>MALKMLTRLQVLTLALFSKGFLLSLGDHNFLRREIKIEGDLVLGGLFPINEKGTGTEECGRINEDRGIQR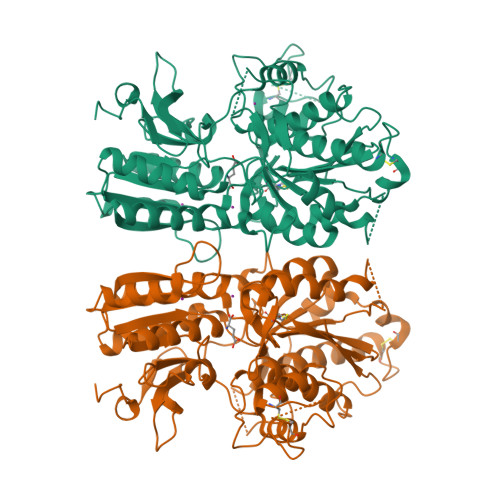LEAMLFAIDEINKDDYLLPGVKLGVHILDTCSRDTYALEQSLEFVRASLTKVDEAEYMCPDGSYAIQENIPLLIAGVIGGSYSSVSIQVANLLRLFQIPQISYASTSAKLSDKSRYDYFARTVPPDFYQAKAMAEILRFFNWTYVSTVASEGDYGETGIEAFEQEARLRNISIATAEKVGRSNIRKSYDSVIRELLQKPNARVVVLFMRSDDSRELIAAASRANASFTWVASDGWGAQESIIKGSEHVAYGAITLELASQPVRQFDRYFQSLNPYNNHRNPWFRDFWEQKFQCSLQNKRNHRRVCDKHLAIDSSNYEQESKIMFVVNAVYAMAHALHKMQRTLCPNTTKLCDAMKILDGKKLYKDYLLKINFTAPFNPNKDADSIVKFDTFGDGMGRYNVFNFQNVGGKYSYLKVGHWAETLSLDVNSIHWSRNSVPTSEGHHHHHH[3x]> DANFRVLSQQLSRLNKTLAAGRPTINHPTFVGSERCRPGYTFTSITLKPPKIDRGSYYGKRLLLPDSVTEYDKKLVSRLQIRVNPLPKFDSTVWVTVRKVPASSDLSVAAISAMFADGASPVLVYQYAASGVQANNKLLYDLSAMRADIGDMR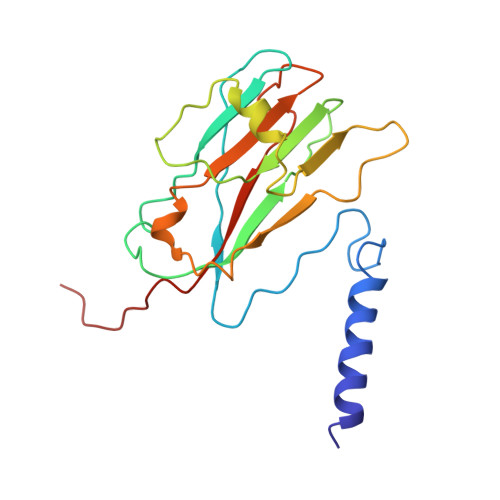KYAVLVYSKDDALETDELVLHVDIEHQRIPTSGVLPV> PRRRDPQDDVYLDITDRLCFAILYSRPKSASNVHYFSIDNELEYENFYADFGPLNLAMVYRYCCKINKKLKSITMLRKKIVHFTGSDQRKQANAAFLVGCYMVIYLGRTPEEAYRILIFGETSYIPFRDAAYGSCNFYITLLDCFHAVKKAMQYGFLNFNSFNLDEYEHYEKAENGDLNWIIPDRFIAFCGPHSRARLESGYHQHSP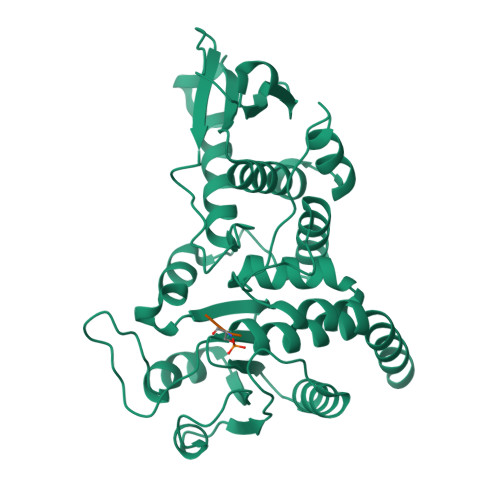ETYIQYFKNHNVTTIIRLNKRMYDAKRFTDAGFDHHDLFFADGSTPTDAIVKEFLDICENAEGAIAVHSKAGLGRTGTLIACYIMKHYRMTAAETIAWVRICRPGSVIGPQQQFLVMKQTNLWLEGDYFRQKLKGQENGQH> GFFLYPHGFYG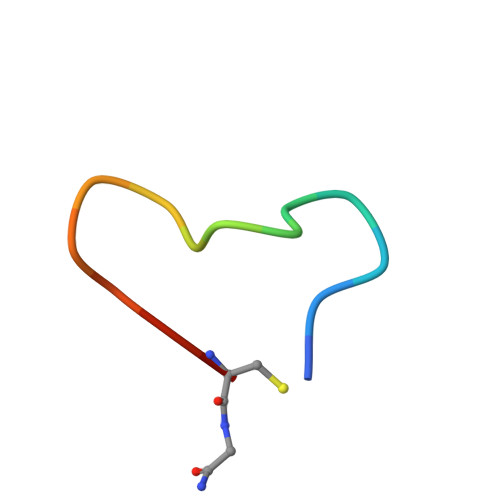IVCX> GUGCGACAAGAAGUUCAGGAAGGGAUUGAGGUGAAAGUCCUCCUCCCGAAUCGUUCAUGGGAGAGUCUAUCCAGACUUGCGUAGCGAGUAAUCGCUAGGUGAGAAGCUCUGGAGACAAUGUACCUGCCCUUCAAUUGGAGGUGCCAGGGCUAGGCUUUGUUCCUAUGGCUAGCGAAAGCGAAUACAGGUUAUUAGGCGUCGUGAAAACAAAACUCUUUCGACAUAAGGGAGAGGCUCGUAGAUGAGUUACCCUCCUUUUUAUGGGGUAACUGAACGAUCAAUAUCUACCGGCGUAGACUGUGAGCCUAAAGGAAACGAAUGAAAGUGUCCCUUCCUGGGAACUUGGUAAGCCCAAUAGACUCCCUCUGGGAAACCAGAGGAGGAGUAAGAGCAAUCUUACUUAUCGUCUAGUGGGUAAAAGACAUAAUAGGAAGCAAAUGCUUGGUUGUAACGAUCGAGAUAGAAUCUGUUGAUUUAAGCUGAAAGGCUGCAGACUUAUUAAAUGGGUGUUCUGCUGUAUGGCGUUCGCGCCUAAGCAGCAGAAUGCGUGAGCCGUGUGCGAUGAAAGUCGCAAGCACGGUUCUGAUGGGGGGAAAACGAGAGAUCGUCUACCUAUCCAAC;> UGUUUAUUAAAAAC

Group II introns are self-splicing ribozymes that catalyze two transesterification reactions to excise themselves from pre-messenger RNA. In the first step of splicing, the 2′-OH of a bulged adenosine residue is used as the nucleophile to attack the 5′ splice site. This is followed by a second step in which the free 3′-OH of the 5′ exon attacks the 3′ splice site to form ligated exons. In group II introns, the 3′ splice site is positioned in the core via domain VI and the IBS3-EBS3 interaction.

The presence of iridium hexammine promotes exon ligation, whereas its absence stalls splicing in crystallo prior to the second step. A comparison of the pre-2s and post-catalytic structures reveals that the basal stem of domain VI, which contains the branch-point adenosine, undergoes a compression in the transition to the second step. In particular, the backbone of the bulged adenosine residue is distorted in the post-catalytic state upon the completion of exon ligation. In addition, the space group and unit cell dimensions remain essentially unchanged between the two states, which is further evidence that these conformational rearrangements are not the result of alterations in crystal packing in the presence and absence of iridium hexammine. The structure of the post-catalytic eukaryotic IIB intron revealed the first evidence for additional junction nucleotides (other than J2/3) participating in base triples within the catalytic triplex. Specifically, the junctions between domains IV and V (J4/5) and domains V and VI (J5/6) are also involved in forming triples at the base of domain V. In comparison with the IIC intron, we observed in the post-catalytic IIB intron that A422 of J2/3 disengages with A551 of the catalytic triad to form a base triple with U549 of J4/5 and U584 of J5/6 at the base of domain V. Surprisingly, the pre-2s structure presented in the current study reveals yet another configuration of the catalytic triplex.The structure of SMURF1 is typical of a NEDD4 subfamily member, with a N-terminal C2 domain for cellular membrane localization, WW domains for target recognition, and a catalytic HECT domain that binds E2 and mediates target ubiquitylation through a surface-protruding catalytic cysteine. At the cellular level, SMURF1 acts as a negative regulator of bone morphogenetic protein (BMP) signaling, which modulates cell migration, proliferation, and apoptosis. Ubiquitin transfer requires a motion facilitated by a flexible hinge that connects the HECT domain N- and C-lobes. To gain structural insights into the mechanism of selective inhibition, we crystallized the HECT domains of both SMURF1 and SMURF2, without and with a representative SMURF1 inhibitor, compound-8 (Cpd-8), and determined structures at 2.05–2.75 Å resolution.

Subsequent X-ray crystallography studies revealed compounds that bind a cryptic cavity distant from the SMURF1 catalytic cysteine. In complex with SMURF1, the inhibitor is buried in an N-lobe cryptic cavity, with only 2% of its surface exposed. Compared with unbound SMURF1, the αH10 of the SMURF1-inhibitor complex is elongated by one and a half turns over the conserved glycine (G634). This shortens the hinge (from 27.0 to 15.4 Å) and replaces G634 at the stem of the flexible hinge with lysine (K637), an amino acid with a lower tolerance of the ϕ/Ψ dihedral angles. The analysis showed that in unbound-SMURF1, I631 of the αH10, along with other nearby residues, occupies the cryptic cavity, preventing small-molecule inhibitor binding. In the presence of Cpd-8, the αH10 is displaced, inducing allosteric elongation. In this altered confirmation, an electrostatic bond is formed between the αH10 D636 and C-lobe R686. R686 is further stabilized by N507, which is allosterically shifted toward R686. The independent mutations D636G, R686A, and N507A did not alter enzymatic activity but conferred resistance to inhibition by Cpd-8, thereby demonstrating the importance of αH10 stabilization of the inhibited form of SMURF1.

> GPDLVQKLKVLRHELSLQQPQAGHCRIEVSREEIFEESYRQIMKMRPKDLKKRLMVKFRGEEGLDYGGVAREWLYLLCHEMLNPYYGLFQYSTDNIYMLQINPDSSINPDHLSYFHFVGRIMGLAVFHGHYINGGFTVPFYKQLLGKPIQLSDLESVDPELHKSLVWILENDITPVLDHTFCVEHNAFGRILQHELKPNGRNVPVTEENKKEYVRLYVNWRFMRGIEAQFLALQKGFNELIPQHLLKPFDQKELELIIGGLDKIDLNDWKSNTRLKHCVADSNIVRWFWQAVETFDEERRARLLQFVTGSTRVPLQGFKALQGSTGAAGPRLFTIHLIDANTDNLPKAHTCFNRIDIPPYESYEKLYEKLLTAVEET>[2x]MKNFYQDGPQLSNTFRSDEALQKILKSLLPADAQKVALPHLEHLGERAVTDMLTWAQEAESQPPVHVPFDPWGRRIDDIKTSHGWKALEKVAAEEGIVATAYDRR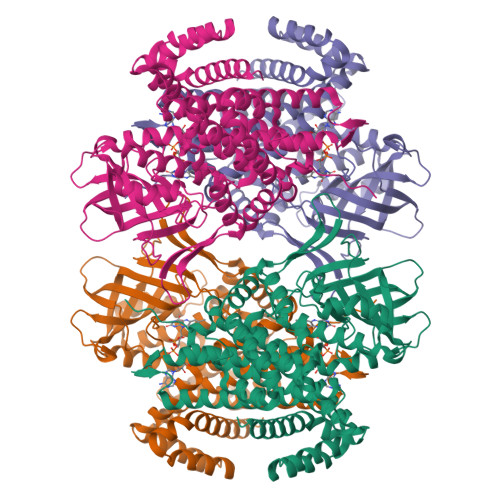FGAASRVYQMALLYLYSPSSAIFSCPLAMTDGAARALELYADADLKARVLPHLLSRDPKTFWTAGQWMTERTGGSDVSGTSTDAHPFTGTSEFGATHSLHGTKWFTSATTSQMALTLARPDGAAPGSRGLSLFFLELRNDKGELNHIQIHRLKDKLGTKALPTAELSLQGTPARMIGGVGEGVKRIASVLNITRIYNSICAVGHIRRALDLAQDYSGKRQAFGKLLKDHPLHKSTLDSLEADFRKCIAFSFFVANLLGQEEVGEASASEKILLRVLTPILKLYTAKKSIHISSEVVEMFGGAGYVEDTGIPRLLRDAQVFSIWEGTTNVLSLDMLRAFEKDQAGQILEQFLVLNEAGSEELVRLQKLLTLSGEQKEQHAREIAFLIGNAVARIAMKKYSL> XCHLEMYDQAKYKPQQASEIFADGASARPLVEHTVARGRLRIDATSTGRVDGDPNGAYVTTIPIRITPELLERGAQRYRIYCAVCHGVN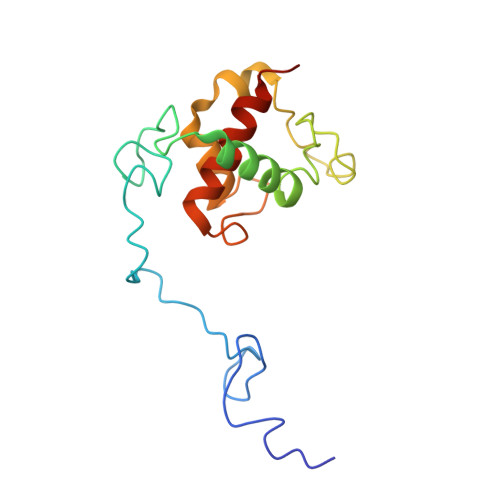GNGRGQVGLLLNPRPPSFYDQRLLDMPDGEYYDVLVNGRRTMYPYGYRVQSISDRWAIVAHIRELQKNPPPQN Here, we report a general and rapid method for discovering α-helically constrained (Helicon) polypeptides that cooperatively induce the interaction between two target proteins without relying on previously known binders or an intrinsic affinity between the proteins. We show that Helicons are capable of binding every major class of E3 ubiquitin ligases, which are of great biological and therapeutic interest but remain largely intractable to targeting by small molecules. In addition to possessing increased stability and membrane permeability, Helicons are capable of binding large, flat protein surfaces that are inaccessible to targeting by small molecules, and Helicons have been developed to target a range of PPI targets in cells and in vivo. Characterizing Helicon-E3 co-structures and mechanisms of action, we identified new binding sites for α-helices on the E3 surfaces, as well as potential probes of the disease-linked E3, WWP123,24, highlighting the generality of our approach against this therapeutically important target class.

We further characterized by x-ray crystallography Helicons derived from these screens. We solved the structure of H314 with the CUL5 N-terminal domain (CUL5NTD) at ~2.8 Å resolution, H313 in complex with VHL-ELOBC at ~3.5 Å resolution, and CUL4B-specific H316 from C77 in complex with the N-terminal domain of CUL4B (CUL4BNTD) at ~2.9 Å resolution. Notably, the co-structure with CUL4BNTD reveals binding to a site that is not biologically relevant since it is not available in the native context of the CUL4B C-terminal domain (CUL4BCTD). This result highlights the importance of biochemical and structural characterization of screening hits to ensure they will be of functional relevance in cells.

>SMPKLPENYTDETWQKLKEAVEAIQNSTSIKYNLEELYQAVENLCSYKISANLYKQLRQICEDHIKAQIHQFREDSLDSVLFLKKIDRCWQNHCRQMIMIRSIFLFLDRTYVLQNSMLPSIWDMGLELFRAHIISDQKVQNKTIDGILLLIERERNGEAIDRSLLRSLLSMLSDLQIYQDSFEQRFLEETNRLYAAEGQKLMQEREVPEYLHHVNKRLEEEADRLITYLDQTTQKSLIATVEKQLLGEHLTAILQKGLNNLLDENRIQDLSLLYQLFSRVRGGVQVLLQQWIEYIKAFGSTIVINPEKDKTMRQELDDFKDKVDHIIDICFLKNEKFINAMKEAFETFINKRPN[4x];>[4x]XDPADRWCELAAWTCDTFX1,4,7,10,13-pentaoxacyclopentadecane | C10 H20 O5 | 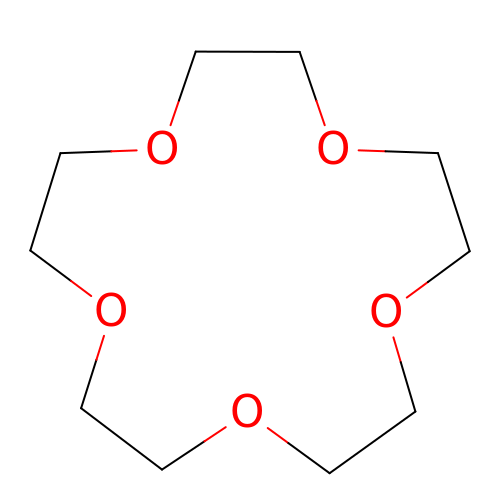VFTFKUDGYRBSAL-UHFFFAOYSA-N We determined the crystal structures of three binary complexes of RPH from L. monocytogenes (RPH-Lm): RPH-Lm·Mg2+·ADP, RPH-Lm·RIF and RPH-Lm·RIF-phosphate (inactivated RIF; RIF-P). The structure of RPH-Lm reveals that the enzyme features a three-domain architecture including an N-terminal ATP-binding domain followed by a large central domain that binds RIF (the RIF-binding domain/RIF-BD), and a smaller C-terminal domain. While numerous examples of antibiotic kinases have been reported, our structural and molecular studies of RPH reveal that these enzymes are distinct from any known antibiotic kinase and therefore represent a class of enzyme with an unusually wide distribution in bacterial genomes, and a complex catalytic mechanism. Crystallography, small-angle scattering, mutagenesis and enzyme characterization showed that the catalytic basis of RIF modification is complex, involving a two-stage mechanism, with transition of a small C-terminal swivel phosphohistidine domain between two active centres.

The ATP-binding domain (residues 1–314) has a fold characteristic of ATP-grasp enzymes. The ATP-grasp fold is comprised of two α/β domains that simultaneously bind an ATP molecule between them. Notably, in the absence of ADP, the ATP-grasp domain is largely disordered and in the absence of RIF, regions of the RIF-BD are disordered. The polyphosphate moiety of ATP is positioned by a subset of amino acids, with Arg117 and Thr136 implicated in binding the α-phosphate, an observed interaction between Mg2+ and the α-β phosphodiester oxygen and coordination of the tri-phosphate by Lys22. Finally, in the RPH-Lm·Mg2+·ADP structure, Glu297 appears to be coordinating the catalytic Mg2+ ion. However, replacement of this residue for Ala had no effect on RIF resistance in vivo and the mutant enzyme was catalytically competent towards both reactions in the ATP-grasp and the RIF-BD. Since Mg2+ ought to be tightly bound to ATP, these results reveal that Mg2+ coordination by Glu297 is not necessary for catalysis. In our RPH-Lm structures, the β-phosphate of ADP and the phosphate on RIF-P are 49 Å apart, implying a significant conformational movement involved in RPH-Lm catalytic activity.

> MKPYVLKFQEIRPHSEALVGGKGMNLGACSNIEGVHVPAGFCLTTEAYKRTLAENNEFTQLLQRLSSLKTSDMDAIREISETIRTLIQHTQIPSEIASYMDATLLDVGGYEMPFAVRSSATAEDLPHASFAGQHDTYLNIIGKDALLQHISMCWASLFTERAIIYRIQNQFDHRKVQLAVVIQQMISPEASGILFTADPITSNRKSLSIDASFGLGEALVSGLVSADSYTVRENTITNKIIATKKLAIYSLKEGGTETRILEKSQQTKQTLTDQQIIQLAKLGRKIEAYFGKPQDIEWCLAEGAFYIVQSRPITTLYPIPEVNEPGNRVYISVAHQQMMTDAMKPLGLSFYLMTTPATMYTAGGRLFVDITQSLSAKVSRDMMVNSLGQSDPLIKDALLTVINKKGFLPPLPTEENPSHATVSGKPPVRSIPDSSSVFELVRNSENSIKHLKQSIETKSGSDLFDFIVEDLEELKRVLFNPTSIDAIMAGMDASAWLNEHIYQWLGEKNVADKLSESAPNNITSQMGLELLDVADVIRPYPAVRAYLEQTKNPDFMNELATLEGGAETKKALEDYLQKYGMRCAGEIDLTKTRWIENPLTLIPLILSNIKNFDSSASMHKFAQGEKEAFHKEQEILRRLQELPDGEQKAMETKEKIDILRHFIGYREYPKYGMINRYFIYKLALLRAGEQLVKDGILQEHEDIYFLYFEELREVVRTGQVDYELINARKRDFATFEKLTPPRILTSDGEMINGEYKRENLPKDAILGLPVSSGTVEGRARVILEMEKADLEDGDILVTAYTDPSWTPAFVSIKGLVTEVGGLMTHGAVIAREYGLPAVVGVENATTIIKDGQQIRINGTEGYIEILD> MSVVSQVILQADDQLRYPTSGELKGIQAFLTTGAQRIRIAETLAENEKKIVDQAQKQLFKKHPEYRAPGGNAYGQRQYNQCLRDY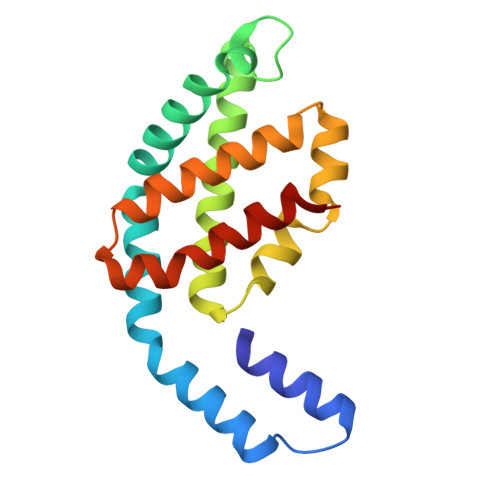GWYLRLVTYGVLAGNKEPIETTGLIGVKEMYNSLNVPVPGMVDAVTVLKDAALGLLSAEDANETAPYFDYIIQFMSHHHHHH methyl 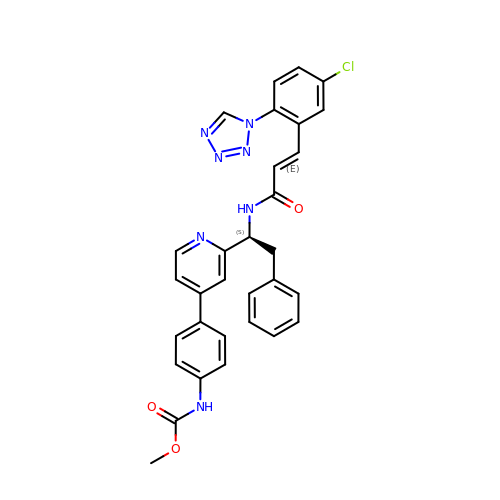~{N}-[4-[2-[(1~{S})-1-[[(~{E})-3-[5-chloranyl-2-(1,2,3,4-tetrazol-1-yl)phenyl]prop-2-enoyl]amino]-2-phenyl-ethyl]pyridin-4-yl]phenyl]carbamate | C31 H26 Cl N7 O3 | ZBUQQUJRHVSUJI-CWBDRXANSA-N>MAHHHHHHMNTDERYKLLRSVGEECIQESELRNLIEKKPLIRCYDGFEPSGRMHIAQGIFKAVNVNKCTAAGCEFVFWVADWFALMNDKVGGELEKIRIVGRYLIEVWKAAGMDMDKVLFLWSSEEITSHADTYWRMVLDIGRQNTIARIKKCCTIMGKTE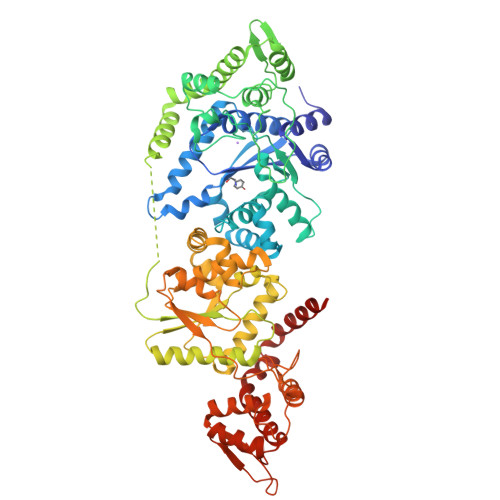GTLTAAQVLYPLMQCCDIFFLKADICQLGLDQRKVNMLAREYCDLIGRKLKPVILSHHMLAGLKQGQAKMSKSDPDSAIFMEDTEEDVARKIRQAYCPRVKQSASAITDDGAPVATDDRNPVLDYFQCVVYARPGAAATIDGTTYATYEDLEQAFVSDEVSEDALKSCLIDEVNALLEPVRQHFASNEEAHELLEAVKSYRKDGATLPLAETALPAAPAKPHACMWMPALLKVPLDVAEGMIKVTKDFIAAHPEGTVTLVLPDWSAVASDEITGVEKDISAALQVNCALLKAYGLPSSVKIVTENEVILGNCDDFWVSVIGIARKNLLSHVEELYGGEVRNAGQVIAALMRVATALMLSVSHVISTSLDGHINAFAREYTKERIDCVQTLEGRIPALHRPGAAPAVLGADDVLYLDDNDMDIRRKIKKAYSAPNEEANPVISVAQHLLAQHGALSIERGEANGGNVSYNTPEALVADCGSGALHPADLKAAVLQLLLDRSAQARALLNGELKKNMTVLRNAEKKMAKKR[4x]>[4x]KARGNVGFVAGSSYGTGSVWTRNNEV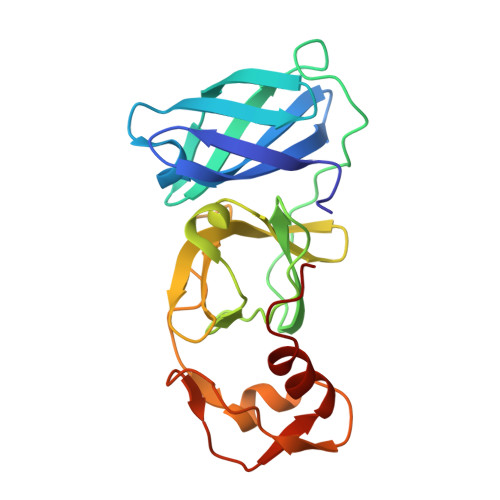VVLTASHVVGRANMATLKIGDAMLTLTFKKNGDFAEAVTTQSELPGNWPQLHFAQPTTGPASWCTATGDEEGLLSGEVCLAWTTSGDSGSAVVQGDAVVGVHTGSNTSGVAYVTTPSGKLLGADTVTLSSLSKHFTGPLTSIPKDIPDNIIADVDAVPRSLAMLIDGLSNRE> MGRKKIQIQRITDERNRQVTFTKRKFGLMKKAYELSVLCDCEIALIIFNHSNKLFQYASTDMDKVLLK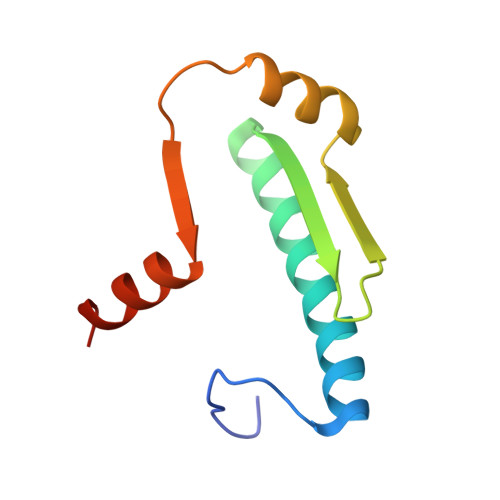YTEYNEPHESRTNADIIETLRKKGFNG The transcriptional activator PrfA, a member of the Crp/Fnr family, controls the expression of some key virulence factors necessary for infection by the human bacterial pathogen Listeria monocytogenes. Structurally, each monomer of PrfA comprises an N-terminal eight-stranded β-barrel domain connected by an α helix linker to a C-terminal α/β domain (Eiting et al., 2005, Vega et al., 2004). The C-terminal region contains the winged helix-turn-helix (HTH) motif responsible for binding to consensus promoter sequences (Eiting et al., 2005, Vega et al., 2004). While most Crp family members require a small molecule cofactor for DNA binding (e.g., cAMP for Crp in Escherichia coli) (Won et al., 2009), PrfA is capable of binding to its DNA consensus sequences with low affinity even in the absence of a cofactor (Eiting et al., 2005).

To understand the structural basis for inhibition, we determined the crystal structure of the PrfAWT-1 complex at a resolution of 2.25 Å. The PrfAWT-1 complex was co-crystallized in the space group P21 where the asymmetric unit contains one biological dimer: monomers A and B. Binding of 1 to PrfAWT was confirmed at two sites, AI in monomer A and BII in monomer B, from difference Fourier electron density maps. Site AI is found at the so-called interdomain tunnel in monomer A, situated between the N- and C-terminal domains. Compound 1 binds with high occupancy at site AI, but no ligand bound to the tunnel in monomer B (i.e., to the BI site). At binding site AI the carboxylate is in close proximity with the charged ɛ-amino groups of Lys64 and Lys122, indicating the potential for both electrostatic interactions and a network of hydrogen bonding, which in the case of Lys122 are mediated through the bulk solvent. The naphthyl ring occupies a hydrophobic part of the tunnel bounded by the peptide backbones of Tyr62, Gln146, Ile149, and Leu150, and the cyclopropyl motif is surrounded between the peptide backbone of Gln123 and the phenyl rings of Tyr63, Phe67, and Tyr126, respectively. The second high-occupancy binding site for compound 1, i.e., the BII site, is found at a hydrophobic pocket in the vicinity of the HTH motif in monomer B. The naphthyl group of compound 1 at site BII is sandwiched between the side chains of four phenylalanines: Phe131 and Phe134 from both monomers in the dimer. At this site the naphthyl group of compound 1 sterically prevents restructuring of residues Phe131 and Phe134 into positions needed for formation of an HTH motif compatible with DNA binding (Levy et al., 2008, Schultz et al., 1991).

>MNAQAEEFKKYLETNGIKPKQFHKKELIFNQWDPQEYCIFLYDGITKLTSISENGTIMNLQYYKGAFVIMSGFIDTETSVGYYNLEVISEQATAYVIKINELKELLSKNLTHFFYVFQTLQKQVSYSLAKFNDFSINGKLGSICGQLLILTYVYGKETPDGIKITLDNLTMQELGYSSGIAHSSAVSRIISKLKQEKVIVYKNSCFYVQNLDYLKRYAPKLDEWFYLACPATWGKLN[2x]> NDKLVELSKSDDNWVMPGKNYDSNNFSDLKQINKGNVKQLRPAWTFSTGLLNGHEGAPLVVDGKMYIHTSFPNNTFALGLDDPGTILWQDKPKQNPAARAVACCDLVNRGLAYWPGDGKTPALILKTQLDGNVAALNAETGETVWKVENSDIKVGSTLTIAPYVVKDKVIIGSSGAELGVRGYLTAYDVKTGEQVWRAYATGPDKDLLLASDFNIKNPHYGQKGLGTGTWEGDAWKIGGGTNWGWYAYDPGTNLIYFGTGNPAPWNETMRPGDNKWTMTIFGRDADTGEAKFGYQKTPHDEWDYAGVNVMMLSEQKDKDGKARKLLTHPDRNGIVYTLDRTDGALVSANKLDDTVNVFKSVDLKTGQPVRDPEYGTRMDHLAKDI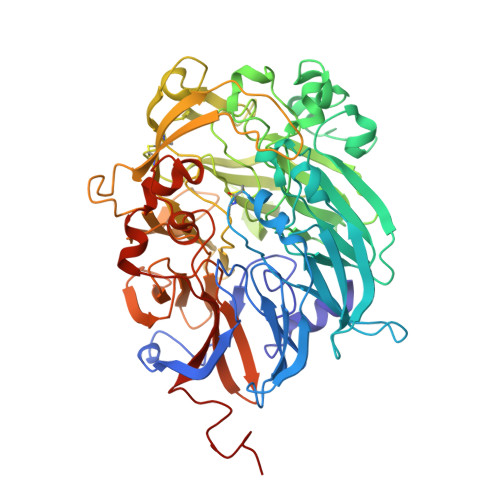CPSAMGYHNQGHDSYDPKRELFFMGINHICMDWEPFMLPYKAGQFFVGATLNMYPGPKGDRQNYEGLGQIKAYNAITGDYKWEKMERFAVWGGTMATAGDLVFYGTLDGYLKARDSDTGDLLWKFKIPSGAIGYPMTYTHKGTQYVAIYYGVGGWPGVGLVFDLADPTAGLGAVGAFKKLANYTQMGGGVVVFSLDGKGPYDDPNVGEWKSAAK At present, the best structurally characterized pLGIC is the G. violaceus ligand-gated ion channel (GLIC), of prokaryotic origin. Each subunit consists of an extracellular domain (ECD), predominantly in a β-sandwich fold, and a transmembrane domain (TMD) composed of four helices, labeled M1–M4. However, the GLIC is a pH-gated channel, activated by lowering the pH, with a maximal activation at pH 4 and a pH50 around 5. We instead found that proton activation is a complex multiple loci mechanism, with the key contribution stemming from the coupling interface between the extracellular and transmembrane domain, with E35 acting as a key proton-sensing residue.

The β9-β10-loop (Loop C) was investigated in conjunction with R133 (Loop B), both of which are located on the principal (+) intersubunit interface, a region that contributes to neurotransmitter binding in eukaryotic pLGICs. In contrast, mutating only the three acidic residues (E177Q-D178N-E181Q) produced a marked decrease in pH50, whereas the individual Asp/Glu residue mutations show Wt-like responses with E181Q having a tendency to decrease the pH50. The mutations E177A and E181A were previously reported in a cinnamic acid study with pH50 values of 5.4 ± 0.1 and 5.6 ± 0.1, respectively, as compared to a Wt value of 5.2 ± 0.1. The decrease in proton sensitivity following neutralization of the E177/D178/E181 cluster, which is completely negated and reversed with the neutralization of the basic R133, K183, and R179 residues, as well as the importance of R179 mutations alone, suggests a role in gating rather than in proton sensing. A structural analysis was performed on E26Q, E26A, E35Q, E35A, E67A, E75A, E82Q, E82A, D86A, D88N, D88A, H127N, E181A, and H277Q mutants, by solving their structure at pH 4. All structures were in the apparently open conformation. There are no significant differences, measured as 5-fold over Wt, seen in the backbone Cα residues of any of the resolved structures, with the exception of E35A and E82Q.

>[5x]GQDMVSPPPPIADEPLTVNTGIYLIECYSLDDKAETFKVNAFLSLSWKDRRLAFDPVRSGVRVKTYEPEAIWIPEIRFVNVENARDADVVDISVSPDGTVQYLERFSARVLSPLDFRRYPFDSQTLHIYLIVRSVDTRNIVLAVDLEKVGKNDDVFLTGWDIESFTAVVKPANFALEDRLASKLDYQLRISRQYFSYIPNIILPMLFILFISWTAFWSTSYEANVTLVVSTLIAHIAFNILVETNLPKTPYMTYTGAIIFMIYLFYFVAVIEVTVQHYLKVESQPARAASITRASRIAFPVVFLLANIILAFLFFGF>[2x]MENKVVEEKQVDKIPLMSPCKMGKFELCHRVVLAPLTRQRSYGYIPQPHAILHYSQRSTNGGLLIGEATVISETG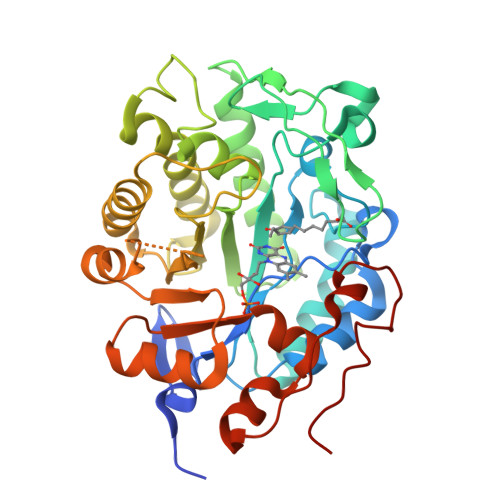IGYKDVPGIWTKEQVEAWKPIVDAVHAKGGIFFCQIWHVGRVSNKDFQPNGEDPISCTDRGLTPQIMSNGIDIAHFTRPRRLTTDEIPQIVNEFRVAARNAIEAGFDGVEIHGAHGYLIDQFMKDQVNDRSDKYGGSLENRCRFALEIVEAVANEIGSDRVGIRISPFAHYNEAGDTNPTALGLYMVESLNKYDLAYCHVVEPRMKTAWEKIECTESLVPMRKAYKGTFIVAGGYDREDGNRALIEDRADLVAYGRLFISNPDLPKRFELNAPLNKYNRDTFYTSDPIVGYTDYPFLETMT> ALVPMVIEQTSRGERSFDIYSRLLKERVIFLTGQVEDHMANLIVAQMLFLEAENPEKDIYLYINSPGGVITAGMSIYDTMQFIKPDVSTICMGQAASMGAFLLTAGAKGKRFCL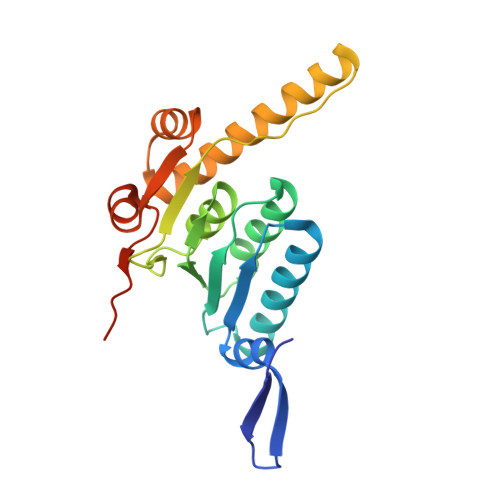PNSRVMIHQPLGGYQGQATDIEIHAREILKVKGRMNELMALHTGQSLEQIERDTERDRFLSAPEAVEYGLVDSILTHRNRSHHHHHH>[2x]MADRIELRGLTVHGRHGVYDHERVAGQRFVIDVTVWIDLAEAANSDDLADTYDYVRLASRAAEIVAGPPRKLIETVGAEIADHVMDDQRVHAVEVAVHKPQAPIPQTFDDVAVVIRRSRRG

The FolB enzyme from Mycobacterium tuberculosis (MtFolB) is a potential target for anti-TB drugs due to its essential role in the survival of the bacillus and the absence of FolB homologues in humans. MtFolB exhibits three activities: aldolase, epimerase, and oxygenase. As an aldolase, this enzyme catalyses the reversible conversion of 7,8-dihydroneopterin (DHNP) to 6-hydroxymethyl-7,8-dihydropterin (HP) and glycolaldehyde (GA) in the folate biosynthesis pathway. Additionally, for MtFolB, the residues Tyr54 and Lys99 play essential roles in the epimerase and aldolase activities of FolB and it is indispensable for the survival of the bacillus.

The crystallographic structure of the FolB enzyme from Mycobacterium tuberculosis (MtFolB), complexed with its inhibitor 8-mercaptoguanine (8-MG), was elucidated at a resolution of 1.95 Å. The crystals diffracted at 1.95 Å resolution and were resolved in the space group P4212, with two MtFolB chains in each asymmetric unit. We found an octamer as the most likely quaternary structure of this complex in solution. Interestingly, Goulding et al. have shown that MtFolB is unique among known FolB enzymes for the fact that the apoenzyme is a tetramer in solution. The octameric structure of MtFolB in complex with 8-MG also presents these major structural changes when compared to the apo-tetrameric form. Loop L1 and the α2a-helix are ordered, while loops L2 and L4 also have shifted positions. Therefore, binding of inhibitor 8-MG to MtFolB induced the major structural changes previously observed upon substrate binding (DHNP), product formation (HP + GA), and complex formation with HP, both in terms of quaternary structure and local rearrangements of loops and helices. 8-MG forms hydrogen bonds with 4 MtFolB residues (Asp53E, Tyr54E, Ile73G and Glu74G). The residues Tyr54E, Ile73G and Glu74G are involved in interactions with all synthesised compounds, as well the 8-MG. Although 8-MG is a non-competitive inhibitor capable of binding to both the free enzyme and the enzyme-substrate binary complex, the crystallographic structure obtained shows that 8-MG binds near the active site of MtFolB.> NLYFQSMSIRDLYHARASPFISLEFFPPKTELGTRNLMERMHRMTALDPLFITVTWGAGGTTAEKTLTLASLAQQTLNIPVCMHLTCTNTEKAIIDDALDRCYNAGIRNILALRGDP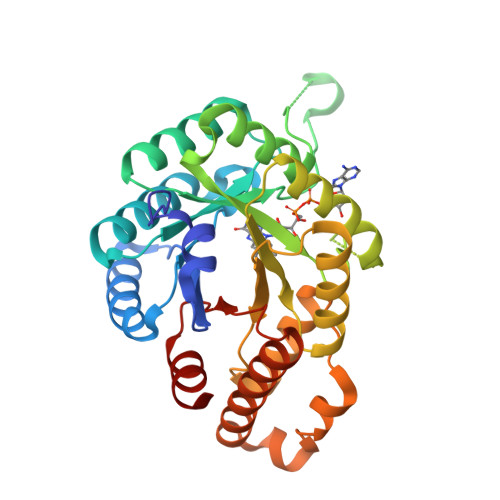PIGEDWLDSQSNESPFKYAVDLVRYIKQSYGDKFCVGVAAYPEGHCEGEAEGHEQDPLKDLVYLKEKVEAGADFVITQLFYDVEKFLTFEMLFRERISQDLPLFPGLMPINSYLLFHRAAKLSHASIPPAILSRFPPEIQSDDNAVKSIGVDILIELIQEIYQRTSGRIKGFHFYTLNLEKAIAQIVSQSP>[4x]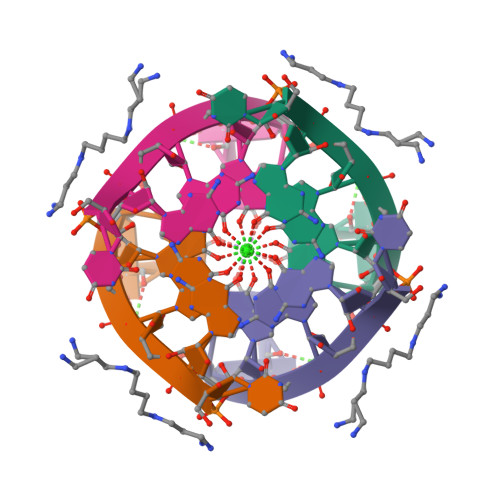UGGGGU ethyl 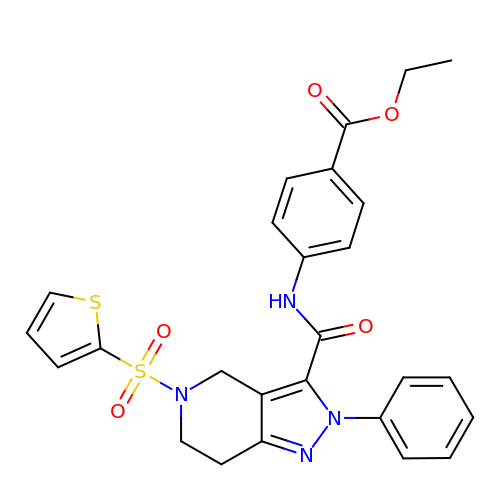4-({2-phenyl-5-[(thiophen-2-yl)sulfonyl]-4,5,6,7-tetrahydro-2H-pyrazolo[4,3-c]pyridine-3-carbonyl}amino)benzoate | C26 H24 N4 O5 S2 | XNXCVMCHZZGPLW-UHFFFAOYSA-N> GSHMLKDSLRPKLS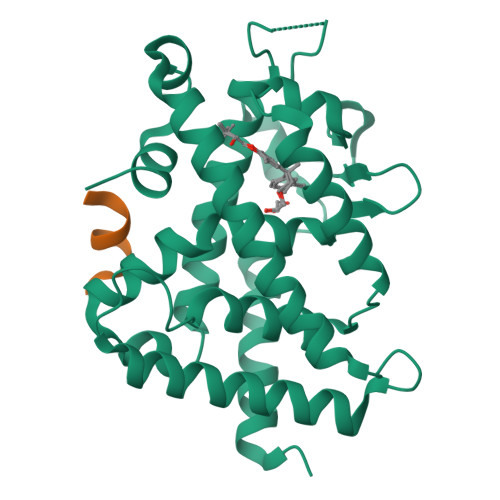EEQQHIIAILLDAHHKTYDPTYADFRDFRPPVRMDGSTGSVTLDLSPLSMLPHLADLVSYSIQKVIGFAKMIPGFRDLTSDDQIVLLKSSAIEVIMLRSNQSFTMDDMSWDCGSQDYKYDVTDVSKAGHTLELIEPLIKFQVGLKKLNLHEEEHVLLMAICIVSPDRPGVQDAKLVEAIQDRLSNTLQTYIRCRHPPPGSHQLYAKMIQKLADLRSLNEEHSKQYRSLSFQPENSMKLTPLVLEVFGNEIS;> KNHPMLMNLLKDN>[4x]SNAMEKIERLRSAFDEAGID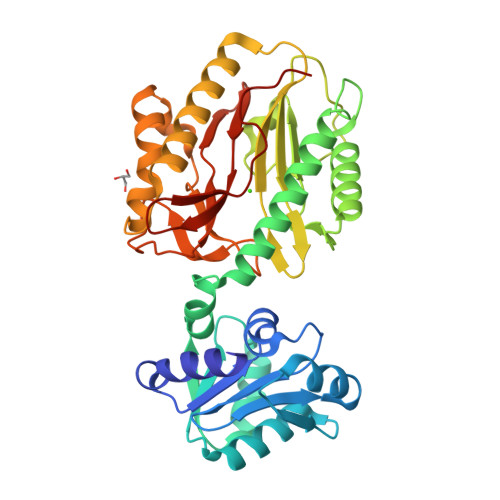GILLTNEHSRRYMANFTGTAGVVLISKKRAQFITDFRYVEQASKQAVGYEIVQHAGLIIDEVAKQVKELGIQKLGFEQDTLTYSSYSAHKEAIDAEFIPTSGLVEKLRLIKTDSEIKILKEAAQIADAAFEHILSFIRPGVSEIEVSNELEFFMRKQGATSSSFDIIVASGLRSALPHGVASEKVIETGDFVTLDFGAYYKGYCSDITRTIAVGEPSDKLKEIYNIVLEAQLRGVNGIKAGLTGREADALTRDYITEKGYGEYFGHSTGHGIGLEIHEAPGLAFRSDTVLEPGMAVTVEPGIYIPGIGGVRIEDDIIVTSEGNEVITKSPKELIIL> KPRNQQQVCPLQNVPAWGYSLYKGIDMSVPLAYDPNNELGDLKDVFPSAVDEMAIGYVCGNPAVKHVLTWKTTDAIQKPIANGDDWGGVIPVGMPCYSKSIRTIKISETENRETEVIDAAPCEYVANMFSYWRAT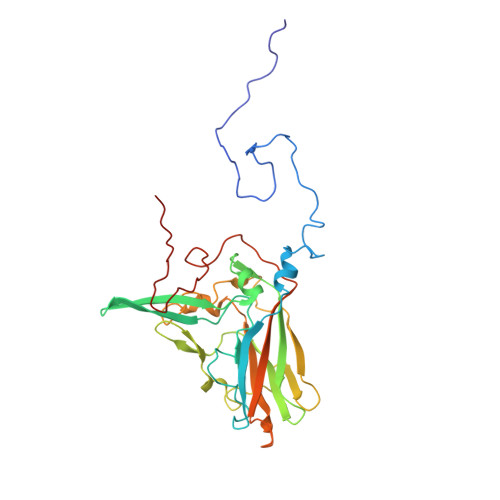MCYRITVVKTAFHTGRLEIFFEPGVIPVKPTVNNIGPDQDQLTGAVAPSDNNYKYILDLTNDTEVTIRVPFVSNKMFLKTAGIYGANSENNWNFHESFSGFLCIRPVTKLMAPDTVSDNVSIVVWKWAEDVVVVEPKPLTSGPTQVYRPPPTASAAVEVLNVELQ> GPSQDPVKLSVSLSDDDVAILDAYVKRAGLP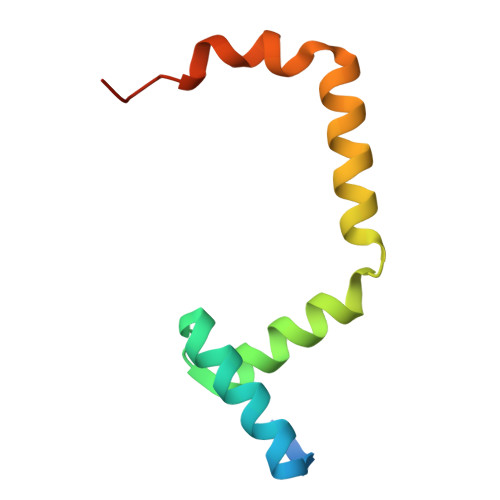SRSAGLQHAIRVLRYPTLEDDYANAWQEWSAAGDTDAWEQTVGDGVGDAPR>[2x]MGPHHHHHHLESTSLYKKAGSENLYFQGMTPGKKIPIFVDGVVLNGPQTDVKAGEKFVEEACRLIMEEVVLKATDVNEKVCEWQPPEQLRQLLDLEMRDTGESQDKLLKLCQDVIHFSVKTNHPRFFNQLYAGLDYYSLAARIITEALNPSIYTYEVSPVFLLVEEAVLKKMIECVGWKEGDGIFNPGGSVSNMCAMNLARYRHCPDIKEKGLSGLPRLILFTSAECHYSMKKAASF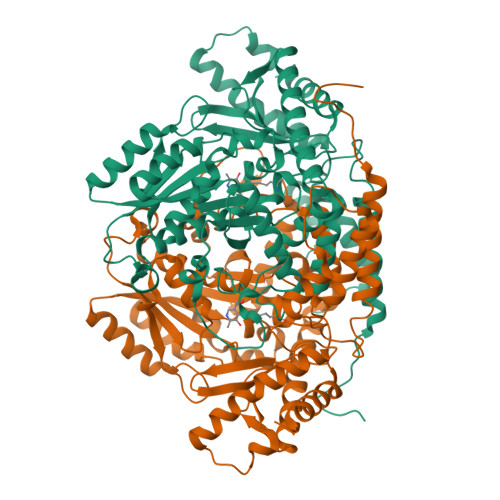LGIGTQNVYFVETDGRGKMIPEDLEKQIWQARQEGAVPFLVCATSGTTVLGAFDPLDEIAEVCERHGLWLHVDASWGGSALVSRKHRRLLHGIHRADSVAWNPHKMLMAGIQCSALLVKDKSDLLKKCYSAKATYLFQQDKFYDVSYDTGDKSIQCSRRPDAFKFWMTWKALGTSGLEERVNRAFALSRYLVDEIKKREGFKLLMEPEYTNVCFWYIPPSLREMEEGPEFWRKLSLVAPAIKEKMMKKGSLMLGYQPHRGKVNFFRQVVISPQVSREDMDFLLDEIDSLGRDM1-(O-CARBOXY-PHENYLAMINO)-1-DEOXY-D-RIBULOSE-5-PHOSPHATE 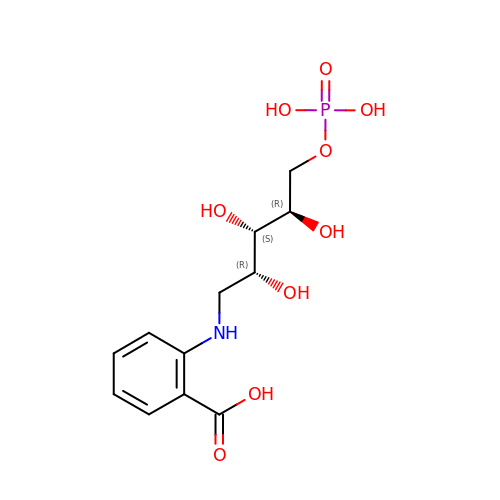| C12 H18 N O9 P | AULMJMUNCOBRHC-MXWKQRLJSA-N> GAASRDDEYDYLFKVVLIGDSGVGKSNLLSRFTRNEFNLESKSTIGVEFATRSIQVDGKTIKAQIWDTAGLERYRAITSAYYRGAVGALLV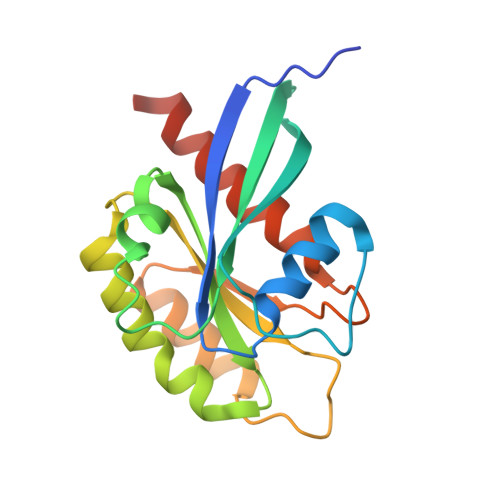YDIAKHLTYENVERWLKELRDHADSNIVIMLVGNKSDLRHLRAVPTDEARAFAEKNGLSFIETSALDSTNVEAAFQTILTEIYRIVSQKQMSDRRE> HHHHHHMSTVQSTAAIPAAYTPGSTFYLPEFPYLLPARRHPASDRIRRSCETWVRANMRFAMADQAEMDALIEEGAALWTCYVLPTADEDRLLNLCRYTEYLSVFDNAMVDRTKIGKDPDAAKELFHRVVNILADRAVGPDFEWGRVLGELWRDMRVGFPEPVWDRFMAEVRRFLSGCVAEITSRSDGMVFDYDTYLKVRRDSVGMGMYFVLGEYGLGIDLTEDLTRHGELREIVDIALEHIMLTNDLFSFRAECAMDDYVNALAVLRLSEGLELQDAVDRLFTVIEGRRTDFMAARRRLESGELGGRADVRAYLDALWHMMAGNLQWSYLTSRYNGIGHVWNNVRSGI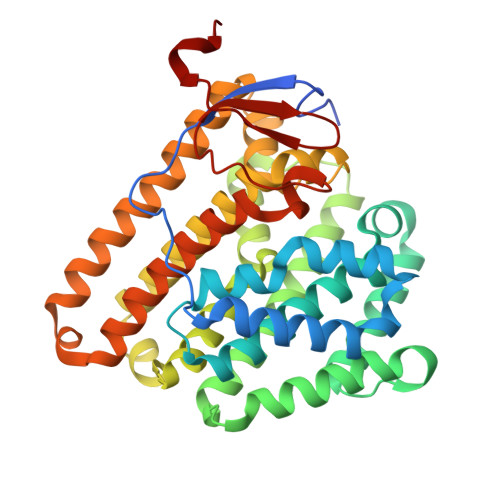VTLHADRTEFSDRPYWSLAR2-[4-[[4-[(3-~{tert}-butyl-1~{H}-pyrazol-5-yl)amino]pyrimidin-2-yl]amino]phenyl]ethanenitrile | C19 H21 N7 | 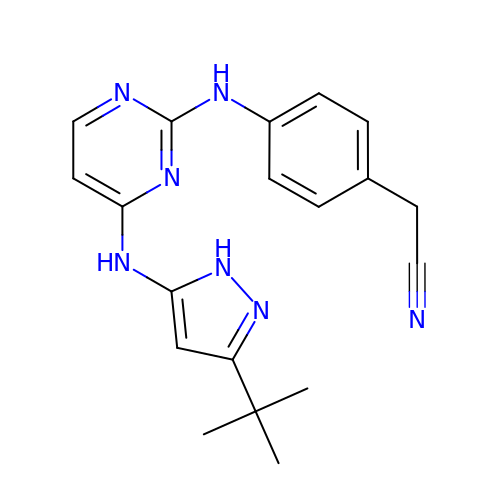HXSSLURGSSMMAH-UHFFFAOYSA-N>[2x]MSTKKKPLTQEQLEDARRLKAIYEKKKNELGLSQESVADKMGMGQSGVGALFNGINALNAYNAALLAKILKVSVEEFSPSIAREIYEMYEAVHHHHHH;> SEELEKA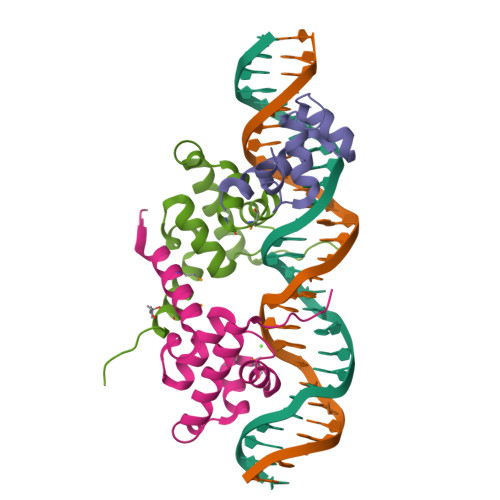LSKLSEREAMVLKLRKGLIDGREHTLEEVGAYFGVTRERIRQIENKALRKLKYHESRTRKLRDFLE>[2x]MRNQDKRAAHKDSEPSTEVNHTASSYQGRQQETGMNLRGIDGNEPTEGSNLLNNNEKMQGTPAEPNHLQRRRQIHACPPRGLLARVITNVTMVILLWAVVWSVTGSECLPGGNLFGIIMLFYCAIIGGKLFGLIKLPTLPPLPPLLGMLLAGFLIRNVPVISDNIQIKHKWSSALRSIALSVILVRAGLGLDSNALKKLK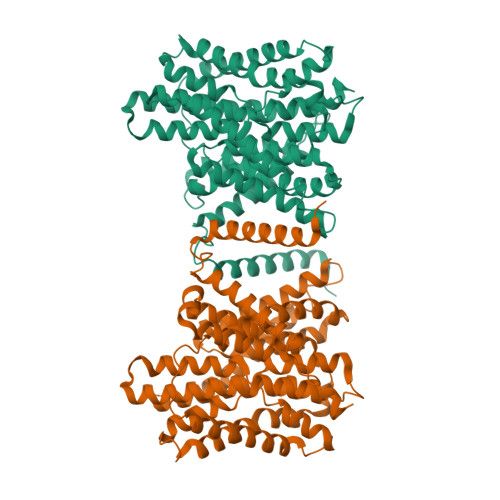GVCVRLSLGPCLIEACTSAVLAYFLMGLPWQWGFMLGFVLGAVSPAVVVPSMLLLQEGGYGVEKGIPTLLMAAGSFDDILAITGFNTCLGMAFSTGSTVFNVLKGVLEVIIGVVTGLVLGFFIQYFPSSDQDNLVWKRAFLVLGLSVLAVFSSTYFGFPGSGGLCTLVTAFLAGRGWASTKTDVEKVIAVAWDIFQPLLFGLIGAEVLITALRPETIGLCVATLGIAVLIRILVTYLMVCFAGFNIKEKIFISFAWLPKATVQAAIGSVALDTARSHGEKQLEGYGMDVLTVAFLSIIITAPVGSLLIGLLGPRLLQKAEQNKDEEDQGETSIQV Signaling by the human C-type lectin-like receptor, natural killer (NK) cell inhibitory receptor NKR-P1, has a critical role in many immune-related diseases and cancer. Human NKR-P1 and LLT1 are type II transmembrane glycoproteins with similar protein topology: an N-terminal cytoplasmic signaling tail, a transmembrane helix, a flexible stalk region, and a C-terminal C-type lectin-like domain (CTLD). In addition, NKR-P1 promotes transendothelial migration to immunologically privileged niches upon interaction with its endogenous ligand, lectin-like transcript 1 (LLT1). Here we report the crystal structures of the NKR-P1 and NKR-P1:LLT1 complexes, which provides evidence that NKR-P1 forms homodimers in an unexpected arrangement to enable LLT1 binding in two modes, bridging two LLT1 molecules.

The asymmetric unit of NKR-P1_glyco contains two monomers, whereas the asymmetric unit of NKR-P1_deglyco contains eight NKR-P1 monomers. All these monomers are arranged into very similar homodimers, with pairwise RMSD on Cα atoms up to 0.5 Å. The dimerization interface of the NKR-P1 homodimer consists of six protein–protein and several water-mediated hydrogen bonds, a peptide bond interaction via delocalized electrons (Lys126-Glu127), and a small hydrophobic core comprising Leu119, Ala120, and Ile168 from both chains. Glycosylation at Asn169 is visible in the electron density maps of both NKR-P1_glyco and _deglyco structures. In NKR-P1_deglyco, a single GlcNAc unit remaining at Asn169 can be well-identified in all eight NKR-P1 chains. Interestingly, the localized first GlcNAc units linked at Asn116 in NKR-P1_glyco and the overlapping GlcNAc units at Asn116 and Asn157 remaining in NKR-P1_deglyco participate in dimerization contacts with residues of helices α1 and regions β2, L1, and β2’ of the opposite subunit of the NKR-P1 homodimer. In NKR-P1_deglyco, density at the homodimer interface can accommodate the remaining GlcNAc unit of either Asn116 of one chain or Asn157 of the opposing chain of the NKR-P1 dimer (for details). Conversely, in NKR-P1_glyco, the first GlcNAc unit at Asn116 is well defined in electron density in both chains, A and B, of the NKR-P1 dimer, while no electron density was found for glycosylation at Asn157. This suggests that although the glycosylation on either Asn116 or Asn157 can contribute to the dimer formation, dimerization might be impaired by steric hindrance if both N-glycans are present simultaneously. However, the structure of the NKR-P1 homodimer shows that Ile168 is found at the dimerization interface rather than at the membrane-distal interaction interface – more specifically, in a small hydrophobic pocket within the dimerization interface.

>ETGGLLNCPIYWQQLREKCLLFSHTVNPWNNSLADCSTKESSLLLIRDKDELIHTQNLIRDKAILFWIGLNFSLSEKNWKWINGSFLNSNDLEIRGDAKENSCISISQTSVYSEYCSTEIRWICQKELTPVRNKVYPDSKHHHHHH[8x]>GPGSMVTSRLFALIPCAGTGSRSGSALPKQYRTLAGRALLHYTLAAFDACSEFAQTLVVISPDDAHFDARRFAGLRFAVRRCGGASRQASVMNGLIQLAEFGATDADWVLVHDAARPGITPALIRTLIGALKDDPVGGIVALPVADTLKRVPAGGDAIERTESRNGLWQAQTPQMFRIGMLRDAIQRAQLEGRDLTDEASA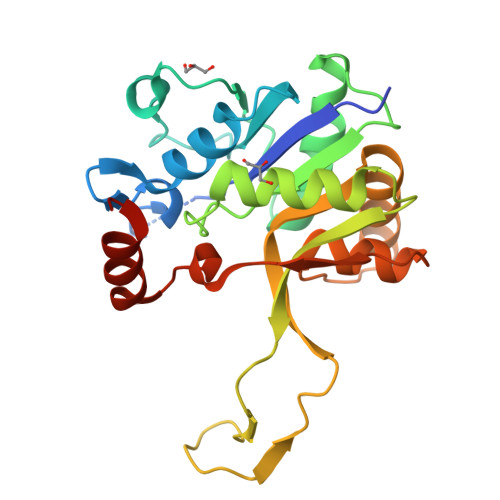IEWAGHTPRVVQGSLRNFKVTYPEDFDLAEAILAHPARAS[4x]>[2x]MISLADLQRRIETGELSPNAAIAQSHAAIEAREKEVHAFVRHDKSARAQASGPLRGIAVGIKDIIDTANMPTEMGSEIYRGWQPRSDAPVVMMLKRAGATIIGKTTTTAFASRDPTATLNPHNTGHSPGGSSSGS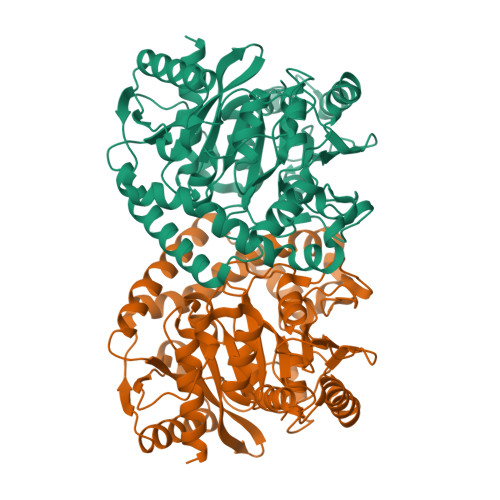AAAVGAGMIPLALGTQTGGSVIQPAAYCGTAAIKPSFRMLPTVGVKCYSWALDTVGLFGARAEDLARGLLAMTGRSEFSGIVPAKAPRIGVVRQEFAGAVEPAAEQGLQAAIKAAERAGASVQAIDLPEAVHEAWRIHPIIQDFEAHRALAWEFSEHHDEIAPMLRASLDATVGLTPKEYDEARRIGRRGRRELGEVFEGVDVLLTYSAPGTAPAKALASTGDPRYNRLWTLMGNPCVNVPVLKVGGLPIGVQVIARFGNDAHALATAWFLEDALAKSG N-methyl-1-(quinoxalin-6-yl)methanamine | C10 H11 N3 | 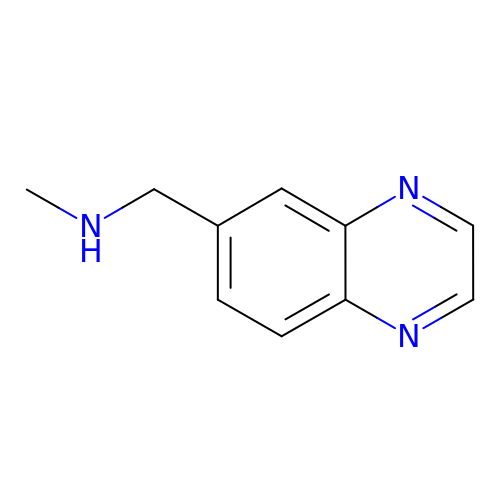QRZKMXOFPHWLCH-UHFFFAOYSA-N>[2x]GDDTDSGENNKDSSIPQGGVTVSPEVLAHRPLIEKYGKEYGIEDYVSYILAIMQVESGGTAEDVMQSSESLGLPPNSLSTEESIKQGVKYFSELLT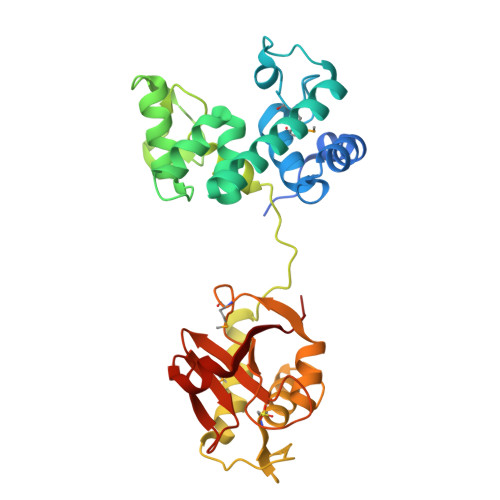SAEQQGVDIDSVIQSYNYGGGFLNYVRSHGKKYTYELAEQFSKEKSGGQKADYPNPIAIPVNGGWRYNYGNQFYVQLVSQYLTDTSPTEFDDETVQVIMDEALKYEGFPYVFGGASPTTSFDCSGLIQWVYDKAGISLPRVAQDQYDATQEISMEEAQAGDLIFFHSTYNAGTYVTHVAIYLEGNRFYHAGDPIGYGDLSSRYWQDHLIGARRVIHN(2R)-2,4-dihydroxy-3,3-dimethyl-N-{3-oxo-3-[(2-sulfanylethyl)amino]propyl}butanamide | C11 H22 N2 O4 S | 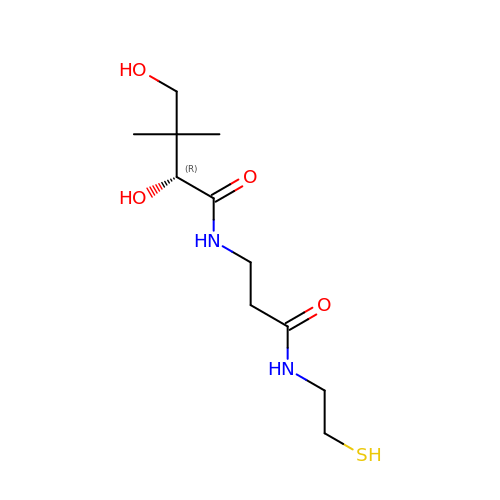ZNXZGRMVNNHPCA-VIFPVBQESA-N> SMNSQPFKLDPKMTHKKLKISNDGLQMEKDESSLKKSHTPERFSGTGCYGAAGNIFIDSGCHYWEVVMGSSTWYAIGIAYKSAPKNEWIGKNASSWVFSRCNSNFVVRHNNKEMLVDVPPHLKRLGVLLDYDNNMLSFYDPANSLHLHTF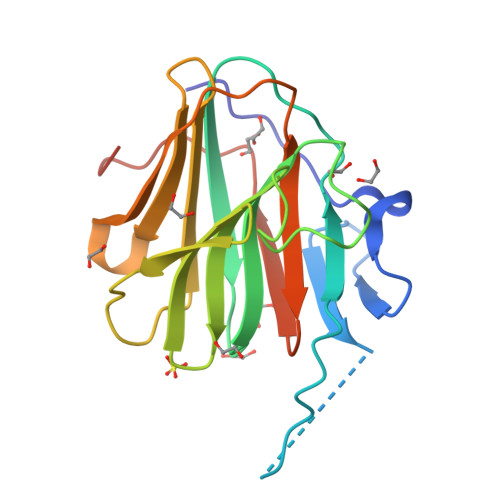DVTFILPVCPTFTIWNKSLMILSGLPAPDFIDYPERQECN> FQGLYAEVKACSSELESLEMELRQQILVNIGKILQDQPSMEALEASLGQGLCSGGQVEPLDGPAGCILECLVLDSGELVPELAAPIFYLLG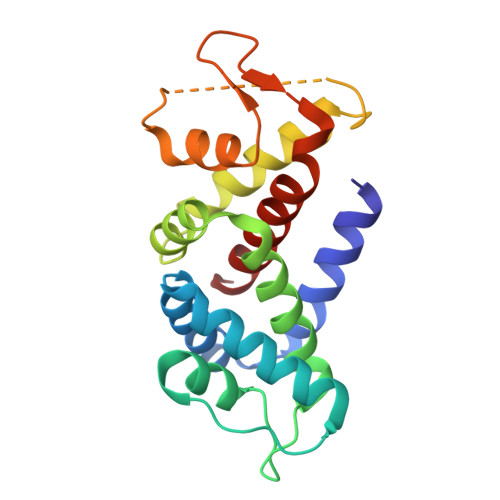ALAVLSETQQQLLAKALETTVLSKQLELVKHVLEQSTPWQEQSSVSLPTVLLGDCWDEKNPTWVLLEECGLRLQVESPQVHWEPTSLIPTSALYASLFLLSSLGQ> ATINNAG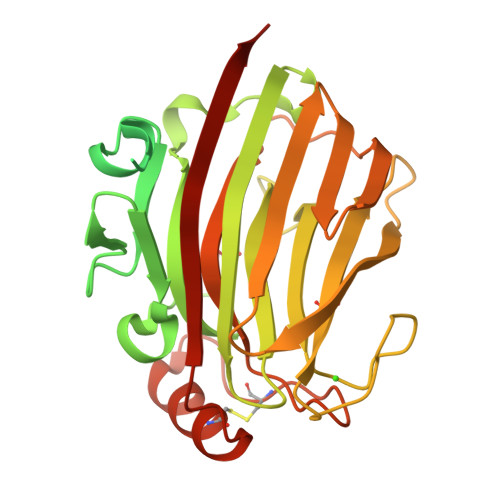FESGFSNWNETDPAAISSDAYSGSKSLKIQGSPARVYQVVDIQPNTEYTLSAYVLGKGQIGVNDLNGLFKNQTFNVSSWTKVTKTFTSANTNSLQVFAKHYNNTSDVRFDNFSLIEGSGSNDGGSDGGSDNSNGSTIPSSITSGSIFDLEGDNPNPLVDDSTLVFVPLEAQHITPNGNGWRHEYKVKESLRVAMTQTYEVFEATVKVEMSDGGKTIISQHHASDTGTISKVYVSDTDESGFNDSVANNGIFDVYVRLRNTSGNEEKFALGTMTSGETFNLRVVNNYGDVEVTAFGNSFGIPVEDDSQSYFKFGNYLQSQDPYTLDKCGEAGNSNSFKNCFEDLGITESKVTMTNVSYTRETNHHHHHH> DNLRHFVQDYAVRALIPYIEHLVAILAEGVTNKKGVSKSLLSATKRWFVTSKPGAGANNQNAVIYTNESAELQTRKLGDLYFMFGHYNLAFQSYHQAKRDFNADSAWQYYAGALEMAALSAFMLGTAQRKTYDYMEDAIVCYLTVCKLQQFATRATLLSMECLKTARLYSEVAKQLIRMTNEESDLRSALLLEQAAYCFLVTQPPMHRKYAFHIVLAGNRYSRAGQRKHAYRCYRQAYQVFQKREWSLAEDHIQYTVAKQAYMLKQLEEASRSFAHLLRPGSLQSAQQQTSFLKEYIQTQNELVKRS;> MTMDATALPSELLVTPQPLVGFCGLDTARVSVHKAVWEAFSGSLQRKAADRAAVQYKLLPPNYEFPVAKPKRASYEWYHPKGILKRNWMLKHLHVLPSVVVLFQDMEWNDLQWTEKQVQCAAIVQALKNTLQERNTRLCLVLLQRAAPLPPGEDLLAAERAASLTNACGITSKMLFILPHTEHLTGYALRLESAFLDMAQSYYALMSKRIRNHRDQLTAAHTSLKIRHQFKLGFVAEMRQDFSTGQKHYFQAYANLDEIRINDGNCLEIKTLAGFLNYKICRLMFKLKTPRDAINQFIIHVEKHKSRVGFKDLAFEHHAWLSTQHSVFAELFCEAIKNGLPALQTQHPGIYYHKAAEFVMKRRDAAMEAYAAMQASSEATPTPIQNPLSLYTEFFGIRAVKTGDLVAEQQANMQLCDQERSYNHSAAIIALLSQAMAQFKIYKCLRFRKKLAIDMAEEYLKSGDHAKALTLYSLMLPDYRQEKWTTIFTDVLLKTLRCAL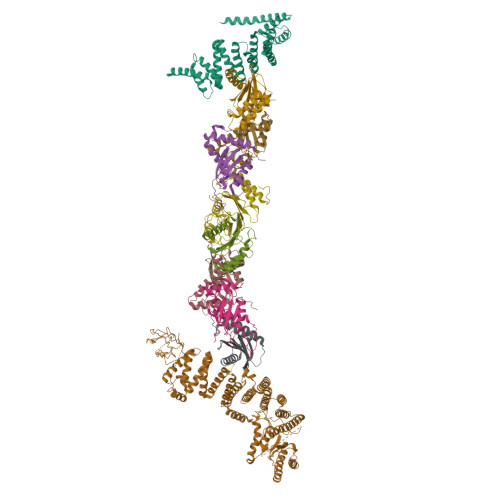LSGSVADYIACSVEALSLRHQSDQSERILILENLWQVFQGVPPMPKTQLTPEAQALWTSALANVKSPIQIDLDKVNDVVEMCATFERVQLSNDDLLQLQLIVRVLTDIPLRIRSFHVILADAGNPQNSYKLEALKYFCFPTLTQLRGQKQPDDEQLENPSQEPKNFEKNMRLEPGSYYQLFCSTEAQQFHENTQLRIVRLEAHMGTDQVAALLTCSSN;>[2x]MSRQASRLDAKKVNSEFLTLTYGALVTQMLRDFENAEDVNKQLERIGYNMGMRLIEDFLARTSAPRCLEMRETADRIQQAFRIYLNIQPTISNWSPASDEFSLVFDSNPLTEFVELPPDLTNLRYSAILSGCIRGALEMVQLEVQCWFVQDQLKGDNVTELRVKFVRRLEEVIPAGED;> MSEEILFDCLHAEIVNYCLDSNKEHDLATLEYIGFTTGYRLIERLTREVSRFKDELETMKFICTDFWMLIYKKQVDNLRTNNHGMYVVQDKAFRFLTRISPGTKQLEHAPKFVAFTCGLVRGALSNLGINSTVTAEVQSIPACKFHIEVNRN;> MTIFNLYIFDKFGTLLHYAEWNRTKKSGITREEEAKLTYGMLFSIKSFVSKISPHDPKEGFLYYKTNRYALHYLETPSGLKFVLNTDTTAINVKELLQQLYAKVWVEFVVRDPLWTPGTVVTSELFQSKLDEFVRQSPIFGIRNI;> MIIYGVYIVSKSGGLIFNLDNNVPRIEHEKTFTYPLDLVLDYDSKKVSVSFNRKDGINVGHVLVAVNGMPVNGVTLDDGRDVRTTLDAPENYPINLKFSRPKMTTNEKIFLASMFYPLFAIASQLSPEPKSSGIEILEADTFTLHCFQTLTGIKFIIISETGLNGIDLLLRKVYELYSDYVLKNPFYSLEMPIRCELFDNKLQELLAQVEKTGISNIDK;> MSTYYFVIVGQNDNPIYEKEFSTVNKELRKEDHRHLTQFIAHAALDLVDEHKWKTANMQLKSIDRFNQWFVSAFITASQIRFIIVHDNKNDEGIKNFFNEMYDTYIKNSMNAFYRINTPIKSPMFEKKSEIFGRKYLLS;> MEKLEALKISSMRPRSNILDRPLSKGKTEVSQSIVALLFSEIVQYSQSRVFTVPELQTRLHDLGQDVGTRIIDLYFVRERSSKRETKLTQMLLFVKTTVWKNLFGKEAEKLEHANDDERTYYIIEKEPLVNTFISVPKDKGSLNCANFTAGIVEAVLTNCGFPCKVTAHWHKGTTYMVKFEDFVIARDKQMEEK;> MAFCIAVIGKDNAPLYLTTSDMEQELELQYHVNAALDVVEEKCLIGKGAPESKELYLGLLYSTENHKIYGFVTNTRVKFIVVIDSSNVALRENEVRAIFRNLHLLYTDAICNPFYIPGESLTSKKFDRAVQKLMSGTA> MKEYTLDKAHTDVGFKIKHLQIS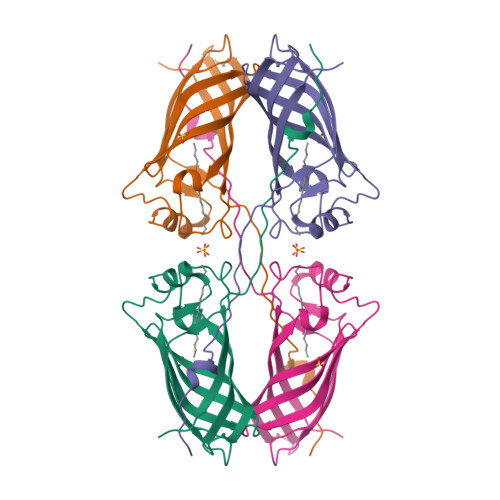NVKGCFKDYSAVIDFDPASAEFKKLDVTIKIASVNTENQTRDNHLQQDDFFKAKKYPDMTFTMKKYEKIDNEKGKMTGTLTIAGVSKDIVLDAEIGGVAKGKDGKEKIGFSLNGKIKRSDFKFATSTSTITLSDDINLNIEVEANEKEGGSHHHHHH> VVGGTEAQRNSWPSQISLQYRSGSSWAHTCGGTLIRQNWVMTAAHCVDRELTFRVVVGEHNLNQNDGTEQYVGVQKIVVHPYWNTDDVAAGYDIALLRLAQSVTLNSYVQLGVLPRAGTILANNSPCYITGWGLTRTNGQLAQTLQQAYLPTVD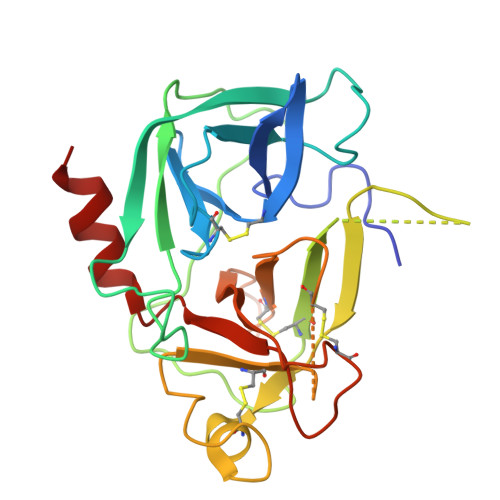YAICSSSSYWGSTVKNSMVCAGGDGVRSGCQGDSGGPLHCLVNGQYAVHGVTSFVSRLGCNVTRKPTVFTRVSAYISWINNVIASN> GQDNTKKEANASNNALKDEKNNENLMEQDFKVPYTDAINIFKDKYKDADIVDLSLERDLNKFVYTVEGVDDNNEYKMKIDANTKDVLEDKTEKL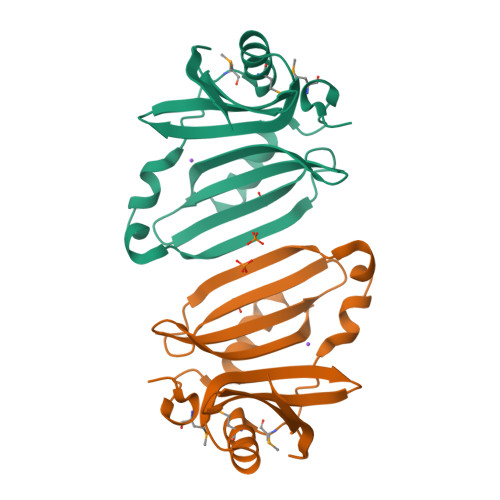DSEDLNGVARKEKLDLNDIMTPQQAMEIALKEQNGIVKEWSLDKDLDVTFYKIRIDKDKNEYDIKVDSKKGTVLKVEKED>MNHKVHHHHHHIEGRHMYSPDRRAALNSVANMVSDNADKDLRYGGLVHDLLADSGKATPNSDAMEDAFGTWTYQELLNHSQAFSAWLDGKGVARGERIVVQLPNIRQTVAVFYGACRRGVVFVPLNPGMKPFHLRSVIADADPRLVIAEDETAADRLRDVTDLPVYSIDSLWADVERLRDAGAGAEAVEVSPEDLAVLIYTSGSTAAPKAVACPHQQIVFAASSINAVL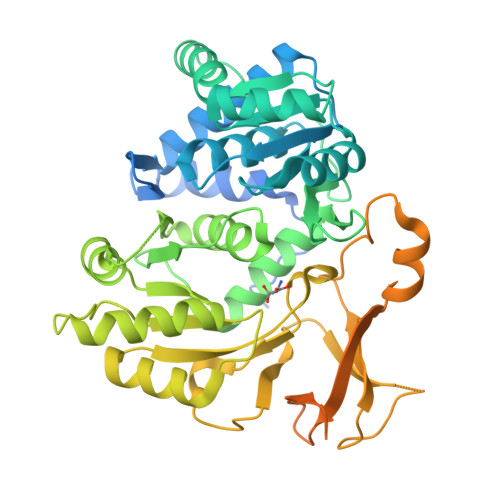GYHAEDIVFCRMSVSWDFGLYKVLISTLTGAKLVLAGGEPDIALVKSLRESGATMMPIVPSLASMLTTLIRRDPEGAPTLRMFTNSAAALPQVTIDALRSAFPGAQVVRMYGQTECKRISIMPPHLEHERPDSVGLPLPGTTIEILDEDGTLLPPGEPGEITVTGPHVMAGYWRAPEITARAYRRDETTGAMRLHTGDYGHLDEDGFLYFGGRRDDMFKRKGTRMSTVEIEAAALDIPGVTAAVALPPTATRDLALCVASDLEPHDVLRSLAERLEPAKVPATCRIVNDFPLTLNGKSERKQLARLLDGSDK[2x]6-methoxy-N-(1-methyl-1H-pyrazol-3-yl)quinazolin-4-amine 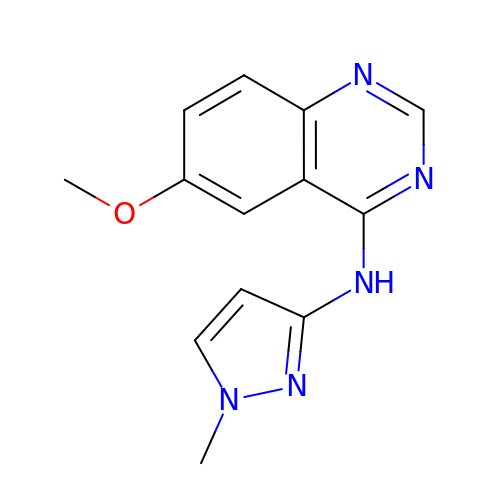| C13 H13 N5 O | BXVGMIRCZUTGFD-UHFFFAOYSA-N>[2x]GVTELSDAQKKQLKEQQEMQQMYDMIMQHKRAMQDMQLLWEKAVQQ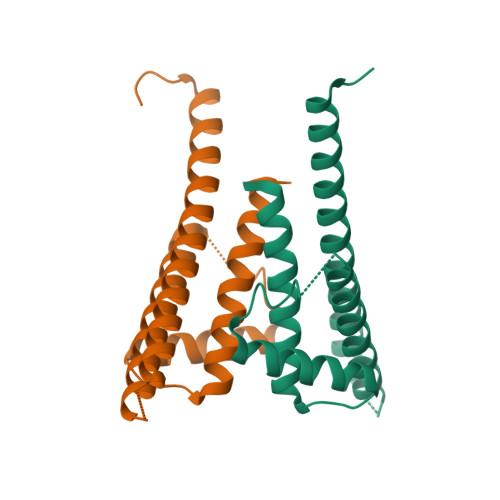HQHGYDSDEEVDSELGTWEHQLRRMEMDKTREWAEQLTKMGRGKHFIGDFLPPDELEKFMETFKALKEGREPDYSEYKEFKLTVENIGYQMLMKMGWKE> MSRGSMEGQGCCGGGGGKTEMIPTEEALRIVFGVSKRLPPVIVSLYEALGKVLAEDIRAPDPLPPYPASVKDGYAVVASDGPGEYPVITESRAGNDGLGVTVTPGTV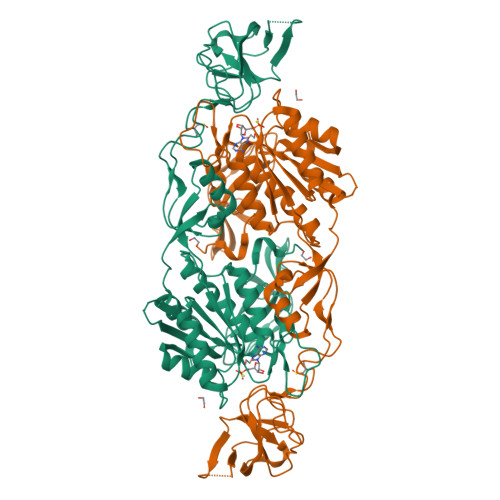AYVTTGGPIPDGADAVVQVEDTKVIGDVSTESKRVKILIQTKKGTDIRRVGCDIEKDATVLTTGERIGASEIGLLATAGVTMVKVYPMPIVAILSTGDELVEPTAGTLGRGQIRDSNRAMLVAAVMQQQCKVVDLGIVRDDRKELEKVLDEAVSSGVDIILTSGGVSMGDRDFVKPLLEEKGKVYFSKVLMKPGKPLTFAEIRAKPTESMLGKTVLAFGLPGNPVSCLVCFNIFVVPTIRQLAGWTSPHPLRVRLRLQEPIKSDPIRPEFHRAIIKWKDNDGSGTPGFVAESTGHQMSSRLLSMRSANALLELPATGNVLSAGSSVSAIIVSDISAFSIDKKASLSEPGSTSGGSAWSHPQFEK> MGSDKIHHHHHHMRLMDILEILYYKKGKEFGILEKKMKEIFNETGVSLEPVNSELIGRIFLKISVLEEGEEVPSFAIKALTPKENAVDLPLGDWTDLKNVFVEEIDYLDSYGDMKILSEKNWYKIYVPYSSVKKKNRNELVEEFMKYFFESKGWNPGEYTFSVQEID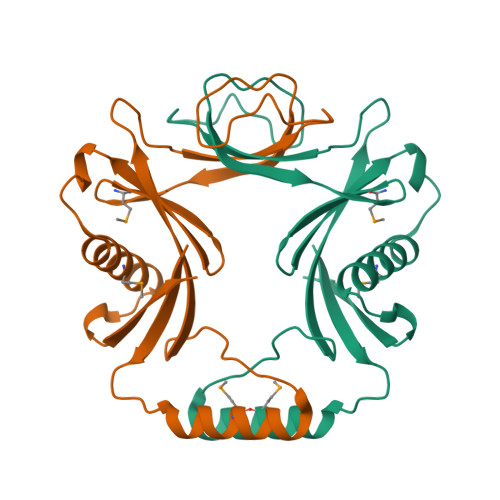NLF> GSSMGSDEQRRELEEKIKLKLEELKTKSEEERKEIKLRVIAYVLVQLEDLQKNLSDEQRRELEEKIKAKLEELKTKSEEERKEIKLRVIAYVLVQLEDLQKNLSDEQRRELEEKIKWKLEELKTKSEEERKEIKLRVIAYVLVQLEDLQKNLS

Deeply knotted proteins, whose topologies may introduce substantial barriers to folding, thus represent an interesting test case for protein design. Here we report our attempts to design proteins with trefoil and pentafoil knotted topologies. We extended previously described algorithms for tandem repeat protein design in order to construct deeply knotted backbones and matching designed repeat sequences (N = 3 repeats for the trefoil and N = 5 for the pentafoil). We developed an approach for designing tandem repeat proteins that fold into a class of knotted topologies known as torus knots.

While kcTRP3c.1 and 3c.2 remained recalcitrant to crystallization, crystals of kcTRP3d.1, 3d.2, and 3d.3 grew readily, and their structures were solved via molecular replacement. kcTRP3d.1 and 3d.3 were phased with the original designed atomic coordinates of kcTRP3d as a molecular probe. The crystal structures of kcTRP3d.1–3 validated the accuracies of the designed molecular models and their intended deeply knotted topologies. Superposition of the structures to the original designed atomic coordinates of kcTRP3d produced all-atom rmsd values of 1.84 Å (kcTRP3d.1), 1.43 Å (kcTRP3d.2), and 1.90 Å (kcTRP3d.3). The structure of kcTRP3d.3 displays 120° rotational averaging in the crystal lattice, such that the positions between the repeating subunits contain a mixture of both peptide loops and protein termini. However, the conformations of secondary structure are unambiguous in electron density. The thermodynamic stabilities of kcTRP3d.1, kcTRP3d.2, and kcTRP3d.3 were studied under equilibrium conditions using the chemical denaturant guanidinium chloride (GdmCl) and unfolding was monitored using both the intrinsic fluorescence and far-UV CD signal of the protein to probe both tertiary and secondary structure. All three constructs show similar stabilities and the stability of kcTRP3d.3 did not change significantly between 25 and 10 °C. Collectively, these data establish that all three constructs unfold and populate an intermediate state, in which a considerable amount, if not all, of the α-helical structure has been lost but in which there remains some burial of the tryptophan side chain(s) suggesting that hydrophobic interactions play a role in stabilizing the intermediate state. As with many knotted proteins, apart from MJ0366 which is both small and has a very shallow knot, the refolding kinetics of kcTRP3d.3 are complex. In contrast to UCH-L1, for kcTRP3d.3 we also have evidence from the interrupted unfolding experiments that the denatured state initially populated on unfolding (which we term D*), undergoes a conformational change over time (with a half-life of ~200–350 ms), which we hypothesize is associated with untying of the knot to the denatured state observed in equilibrium conditions (D).3-hydroxy-5-[5-(6-hydroxy-7-propyl-2H-indazol-3-yl)-1,3-thiazol-2-yl]pyridine-2-carboxylic 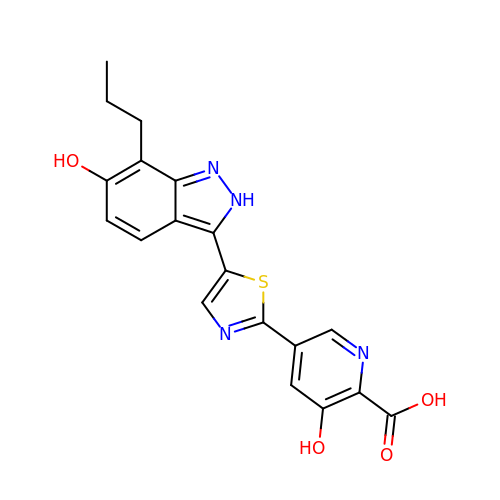acid | C19 H16 N4 O4 S | YZWBQSFGTLQFTB-UHFFFAOYSA-N The Drosophila peptidoglycan recognition protein SA (PGRP-SA) is critically involved in sensing bacterial infection and activating the Toll signaling pathway, which induces the expression of specific antimicrobial peptide genes. PGRP-SA is a secreted protein circulating in the hemolymph (the insect blood) of Drosophila. Members of the PGRP family are expressed as either secreted, cytosolic, or transmembrane forms, which all share a conserved 165-amino acid domain (the PGRP domain) with an evolutionary connection to bacteriophage T7 lysozyme. Contrary to the general belief that PGRP-SA has lost enzyme function and serves primarily for PG sensing, we found that it possesses an intrinsic L,D-carboxypeptidase activity for diaminopimelic acid-type tetrapeptide PG fragments but not lysine-type PG fragments, and that Ser158 and His42 may participate in the hydrolytic activity.

We have determined the crystal structure of PGRP-SA to 2.2-Å resolution and analyzed its peptidoglycan (PG) recognition and signaling activities. The crystal structure was determined by molecular replacement, using the structure of PGRP-LB as a search model. Although the crystals were grown from full-length PGRP-SA (177 residues plus 6×His-tag; residues numbered from the N terminus of the purified polypeptide chain, as determined by N-terminal sequencing), clear electron density was visible only from Cys11 to Pro177. The structure of PGRP-SA reveals a single domain composed of a central seven-stranded mixed β sheet (B1, B3, B4, B5, B7, B8, and B9) flanked by three major helices (H2, H3, and H5), a small two-stranded parallel β sheet (B2 and B6), and two single-turn helices (H1 and H4). The H2 helix contains one turn of rarely observed π helix at its C terminus (residues 64–70). This helix, together with the L1–L4 loops and the central β sheet, forms a prominent extended surface groove, which in PGRP-LB includes a zinc cage. However, PGRP-SA has lost two of the four zinc-coordinating residues present in PGRP-LB; accordingly, the rPGRP-SA crystals exhibit no X-ray absorption at the zinc edge, and we found no electron density for possible metal ions around the groove. PGRP-SA contains two disulfide bridges (Cys11-Cys134 and Cys48-Cys54), whereas PGRP-LB has only one. The most prominent feature of PGRP-SA is a long surface groove demarcated by residues of the H2 helix from one side and of the L1–L4 loops from the other side, with the residues from B3, B4, and B7 of the central β sheet forming the base of the groove. In the PGRP-SA structure the Oγ of the Ser158 residue is positioned within hydrogen-bonding distance (2.95 Å) of the Nδ1 of the highly conserved His42 residue.

>MQPVRFGSPWIMAIGLVLLLLAFVSAGKSRQRSPANCPTIKLKRQWGGKPSLGLHYQVRPIRYVVIHHTVTGECSGLLKCAEILQNMQAYHQNELDFNDISYNFLIGNDGIVYEGTGWGLRGAHTYGYNAIGTGIAFIGNFVDKLPSDAALQAAKDLLACGVQQGELSEDYALIAGSQVISTQSPGLTLYNEIQEWPHWLSNPHHHHHH[2x]>[2x]MSAIENFDAHTPMMQQYLRLKAQHPEILLFYRMGDFYELFYDDAKRASQLLDISLTKRGASAGEPIPMAGIPYHAVENYLAKLVNQGESVAICEQIGDPATSKGPVERKVVRIVTPGTISDEALLQERQDNLLAAIWQDSKGFGYATLDISSGRFRLSEPADRETMAAELQRTNPAELLYAEDFAEMSLIEGRRGLRRRPLWEFEIDTARQQLNLQFGTRDLVGFGVENAPRGLCAAGCLLQYAKDTQRTTLPHIRSITMEREQDSIIMDAATRRNLEITQNLAGGAENTLASVLDCTVTPMGSRMLKRWLHMPVRDTRVLLERQQTIGALQDFTAGLQPVLRQVGDLERILARLALRTARPRDLARMRHAFQQLPELRAQLETVDSAPVQALREKMGEFAELRDLLERAIIDTPPVLVRDGGVIASGYNEELDEWRALADGATDYLERLEVRERERTGLDTLKV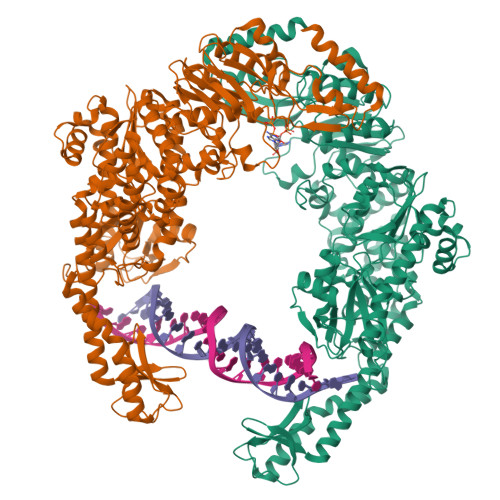GFNAVHGYYIQISRGQSHLAPINYMRRQTLKNAERYIIPELKEYEDKVLTSKGKALALEKQLYEELFDLLLPHLEALQQSASALAELDVLVNLAERAYTLNYTCPTFIDKPGIRITEGRHPVVEQVLNEPFIANPLNLSPQRRMLIITGPNMGGKSTYMRQTALIALMAYIGSYVPAQKVEIGPIDRIFTRVGAADDLASGRSTFMVEMTETANILHNATEYSLVLMDEIGRGTSTYDGLSLAWACAENLANKIKALTLFATHYFELTQLPEKMEGVANVHLDALEHGDTIAFMHSVQDGAASKSYGLAVAALAGVPKEVIKRARQKLRELESISPNAAATQVDGTQMSLLSVPEETSPAVEALENLDPRSLTPRQALEWIYRLKSLV>MLSNSQGQSPPVPFPAPAPPPQPPTPALPHPPAQPPPPPPQQFPQFHVKSGLQIKKNAIIDDYKVTSQVLGLGINGKVLQIFNKRTQEKFALKMLQDCPKARREVELHWRASQCPHIVRIVDVYENLYAGRKCLLIVMECLDGGELFSRIQDRGDQAFTEREASEIMKSIGEAIQYLHSINIAHRDVKPENLLYTSKRPNAILKLTDFGFAKETTSHNSLTTPCYTPYYVAPEVLGPEKYDKSCDMWSLGVIMYILLCGYPPFYSNHGLAISPGMKTRIRMGQYEFPNPEWSEVSEEVKMLIRNLLKTEPTQRMTITEFMNHPWIMQSTKVPQTPLHTSRVLKEDKERWEDVKEEMTSALATMRVDYEQIKIKKIEDASNPLLLKRRKKARALEAAALAH[4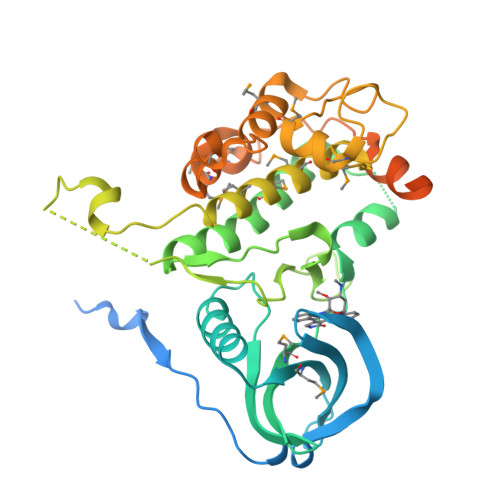x]>[3x]GG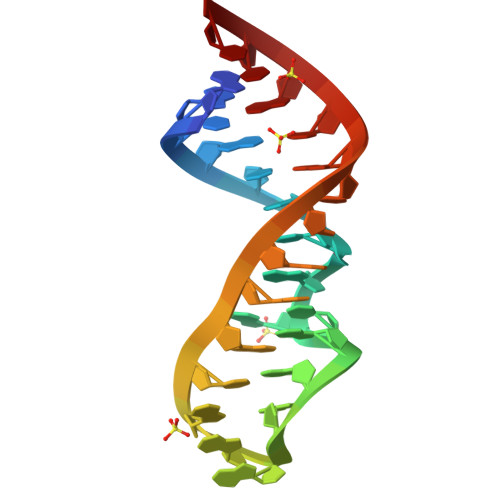UGCUCAGUAGGAGACGAACCGCACC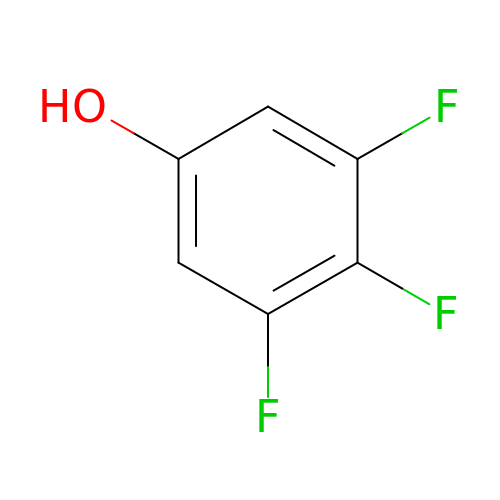3,4,5-tris(fluoranyl)phenol | C6 H3 F3 O | ZRTWIJKGTUGZJY-UHFFFAOYSA-N>[2x]ADFEVHMLN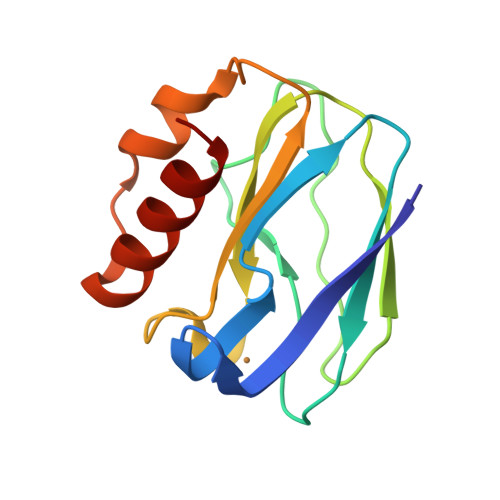KGKDGAIVFEPASLKVAPGDTVTFIPTDKGHNVETIKGMIPDGAEAFKSKINENYKVTFTAPGVYGVKCTPHYGMGMVGVVQVGDAPANLEAVKGAKNPKKAQERLDAALAALGN(2R)-1-[3-sulfanyl-2-(sulfanylmethyl)propanoyl]pyrrolidine-2-carboxylic acid | C9 H15 N O3 S2 | 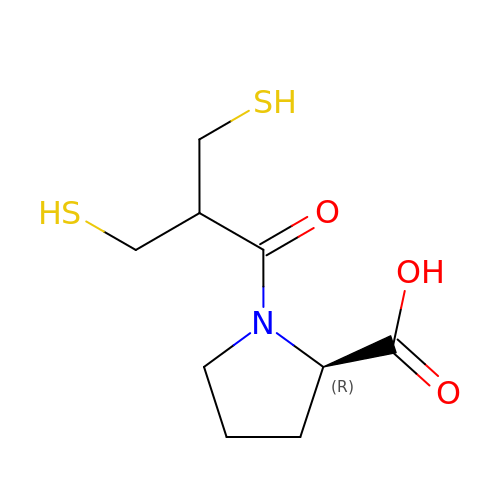CTDDWEHVCFADKZ-SSDOTTSWSA-N>GPPGPPGP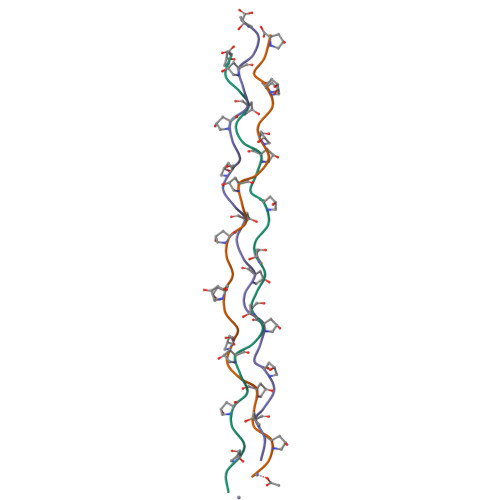PGPPALPGPPGPPGPPGPP[3x]>EFNPYQKGPDPTASALERNGPFAIRSTSVSRTSVSGFGGGRLYYPTASGTYGAIAVSPGFTGTSSTMTFWGERLASHGFVVLVIDTITLYDQPDSRARQLKAALDYLATQNGRSSSPIYRKVDTSRRAVAGHSMGGGGSLLAARDNPSYKAAIPMAPWNTSSTAFRTVSVPTMIFGCQDDSIAPVFSSAIPIYNAIPNSTRKNYVEIRNDDHFCVMNGGGHDATLGKLGISWMKRFVDNDTRYSPFVCGAEYNRVVSSYEVSRSYNNCPY[2x]

Substituting His/Phe with Ser/Ile should expand the substrate-binding pocket to accommodate the bulkier substrate PET, and the strategy termed “double mutation (DM)” has proven to be useful to enhance PET hydrolytic activity of several IsPETase-like enzymes. Here, we report our experience in establishing the P. pastoris strain that expresses a PET hydrolytic enzyme from Caldimonas taiwanensis termed CtPL-DM that was identified from sequence mining from GenBank and modified by the DM strategy. In contrast to the protein expressed in Escherichia coli, CtPL-DM expressed in P. pastoris is inactive in PET degradation. Structural analysis indicates that a putative N-glycosylation site N181 could restrain the conformational change of a substrate-binding Trp and hamper the enzyme action.

We thus proceeded to solve the crystal structure of P. pastoris-expressed CtPL-DM to explore the possible reason underlying the loss of activity. We obtained the apo-form crystal structures of wild type and inactive variant S155A of CtPL-DM, which adopt the canonical α/β-hydrolase fold and are highly identical to the structure of IsPETase (Cα RMSD 0.477 Å and 0.471 Å). The catalytic triad was found in an open cleft formed on the protein surface. The TPA-binding W180 adopts the C-type conformation in the CtPL-DM structure and an alternative type in CtPL-DM-S155A. This suggests that DM strategy has conferred the TPA-binding Trp in CtPL-DM a wobble conformation. In both structures, a sugar that is covalently linked to N220 was observed. Protein sequence analysis indicates that there are three putative N-glycosylation sites in addition to N220 including N168, N181 and N261. N181 and N261 face towards the bulk solvent and could be glycosylated, despite no additional electron density map attached to these residues was observed. Notably, N181 is located adjacent to the TPA-binding residue W180, and its glycosylation, if any, could likely impose spatial hindrance to prevent W180 from wobbling and impact the substrate binding. Nonetheless, W180 in F235L-S155A, which carries N181A mutation, shall be able to wobble freely. On the other hand, the conformational change of W180 in CtPL-DM and CtPL-DM-S155A is restrained by the glycosylated N181, thus impedes the binding of PET.> MADKFAAKFVSHKISRTRWRPVSASSLQQPDVFATGSWDNEENKVCVWATSDFGATSLDEEYQGDPKQLCDIKHPGDVMDMQFLDKERIVTGSSTGTVTIFRHHENNQTLSVNQRWEQAHYHVGSNMRAPCTAIVCSSPEIVSVGEDGRINCFRAESRDVLRTIDDADSSTMHGVT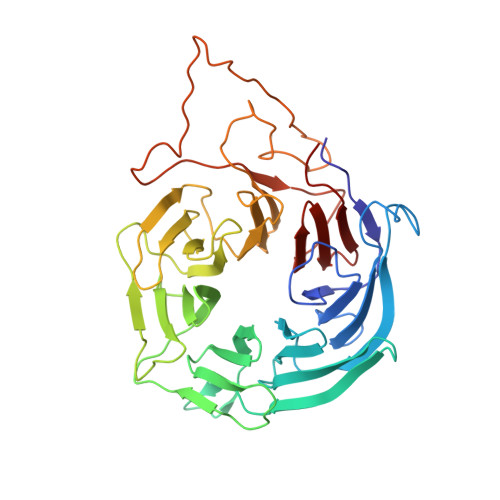FLRTTEILTVNSVGQLKLWDLRKQGNDPTQIFSVTGERVPLHCVDRHPNQQHVVATGGQDGMLCIWDVRHGKMPMSLLNAHEAEMWEVHFHPSNPDHLFTCSEDGSLWHWDASADSEKPTFLLGGRSTFNISRSSIAPPNANQSLACAWLSTDPTKGQLEITNLLPSSTLSVNSLDVLGQNLVCGTDAEAIYVTRRLFS>[4x]AIAMTH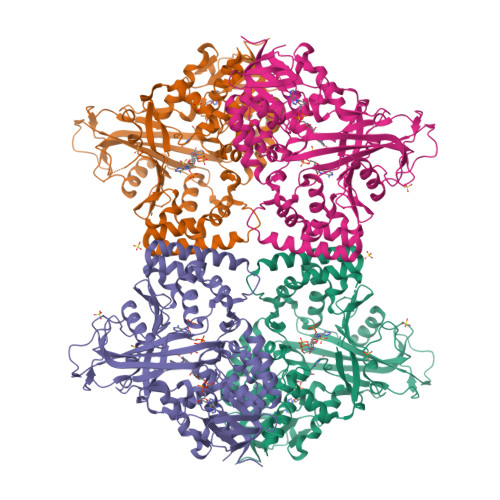PDISVDVLVIGAGPTGLGAAKRLNQIDGPSWMIVDSNETPGGLASTDVTPEGFLYDVGGHVIFSHYKYFDDCLDEALPKEDDWYTHQRISYVRCQGQWVPYPFQNNISMLPKEEQVKCIDGMIDAALEARVANTKPKTFDEWIVRMMGTGIADLFMRPYNFKVWAVPTTKMQCAWLGERVAAPNLKAVTTNVILGKTAGNWGPNATFRFPARGGTGGIWIAVANTLPKEKTRFGEKGKVTKVNANNKTVTLQDGTTIGYKKLVSTMAVDFLAEAMNDQELVGLTKQLFYSSTHVIGVGVRGSRPERIGDKCWLYFPEDNCPFYRATIFSNYSPYNQPEASAALPTMQLADGSRPQSTEAKEGPYWSIMLEVSESSMKPVNQETILADCIQGLVNTEMLKPTDEIVSTYHRRFDHGYPTPTLEREGTLTQILPKLQDKDIWSRGRFGSWRYEVGNQDHSFMLGVEAVDNIVNGAVELTLNYPDFVNGRQNTERRLVDGAQVFAKSKAQ The cytoplasmic F420-reducing [NiFe]-hydrogenase (Frh) belongs to the group 3 [NiFe]-hydrogenases, which catalyze the reversible reduction of the soluble hydride carrier, NAD(P) or F420. Frh is a heterotrimeric enzyme composed of the large subunit FrhA (45 kDa) with a binuclear [NiFe]-center, the small subunit FrhG (26 kDa) with three [4Fe4S] clusters and the iron–sulfur flavoprotein FrhB (31 kDa) with a [4Fe4S] cluster and FAD, and the F420-binding site. The Frh complex is a 1.2-MDa dodecamer with tetrahedral symmetry. Our structure shows that each heterotrimer encompasses a complete electron transfer chain that runs from the [NiFe] cluster in FrhA via the three Fe-S clusters in FrhG and one Fe-S cluster and FAD in FrhB to F420.

We present here the structure of the Frh complex from the hydrogenotrophic methanogenic archaeon, Methanothermobacter marburgensis, by cryo-electron microscopy. To identify the substrate-binding site, we imaged the FrhABG complex in the presence of a large excess of F420, and calculated maps, which were refined to a similar resolution. At all refinement stages, the map showed an additional density in a region that was empty in maps of Frh without substrate. This density runs approximately parallel to the FAD isoalloxazine ring, at a distance of ∼4 Å. We conclude that it represents the isoalloxazine ring of the F420 substrate. It is seated in a large pocket surrounded by highly conserved residues, with easy access to the surface of the complex. The F420 density is close to the small residues S209 and V210 in a loop between two β-strands, which are part of the longest conserved region of FrhB. The location between this ring and the surface of the complex suggests that one or both of the conserved lysines may interact with the phosphate group of F420. The map of Frh in the presence of substrate is similar to the substrate-free map, indicating that F420 binding does not involve major conformational changes. The cofactors describe a curvilinear path in the protein interior, almost parallel to the surface of the complex, with distances of ∼10 Å between neighbors, except FAD and F420, which are in van der Waals contact to enable hydride transfer.

> MSERIVISPTSRQEGHAELVMEVDDEGIVTKGRYFSITPVRGLEKMVTGKAPETAPVMVQRICGVCPIPHTLASVEAIDDSLDIEVPKAGRLLRELTLAAHHVNSHAIHHFLIAPDFVPENLMADAINSVSEIRKNAQYVVDMVAGEGIHPSDVRIGGMADNITELARKRLYARLKQLKPKVNEHVELMIGLIEDKGLPEGLGVHNQPTLASHQIYGDRTKFDLDRFTEIMPESWYDDPEIAKRACSTIPLYDGRNVEVGPRARMVEFQGFKERGVVAQHVARALEMKTALSRAIEILDELDTSAPVRADFDERGTGKLGIGAIEAPRGLDVHMAKVENGKIQFYSALVPTTWNIPTMGPATEGFHHEYGPHVIRAYDPCLSCATHVMVVDDEDKSVIKNEMVKI;> MSLIARIKRFLGLEAEAKREEPEKEKSEPVGASKEEVEKVAEENAKPRIGYIHLSGCTGDAMSLTENYDILAELLTNMVDIVYGQTLVDLWEMPEMDLALVEGSVCLQDEHSLHELKELREKAKLVCAFGSCAATGCFTRYSRGGQQAQPSHESFVPIADLIDVDLALPGCPPSPEIIAKTVVALLNNDMDYLQPMLDLAGYTEACGCDLQTKVVNQGLCIGCGTCAMACQTRALDMTNGRPELNSDRCIKCGICYVQCPRSWWPEEQIKKELGL;> MVLGTYKEIVSARSTDREIQKLAQDGGIVTGLLAYALDEGIIEGAVVAGPGEEFWKPQPMVAMSSDELKAAAGTKYTFSPNVMMLKKAVRQYGIEKLGTVAIPCQTMGIRKMQTYPFGVRFLADKIKLLVGIYCMENFPYTSLQTFICEKLGVSMELVEKMDIGKGKFWVYTQDDVLTLPLKETHGYEQAGCKICKDYVAELADVSTGSVGSPDGWSTVITRTDAGDSIFKQAVEAGLFETKPIEEVKPGLGLLEKLAAQKKEKAEKNIAARKEMGLPTPF>HHHHASILIDTSAWVEYFRATGSIAAVEVRRLLSEEAARIAMCEPIAMEILSGALDDNTHTTLERLVNGLPS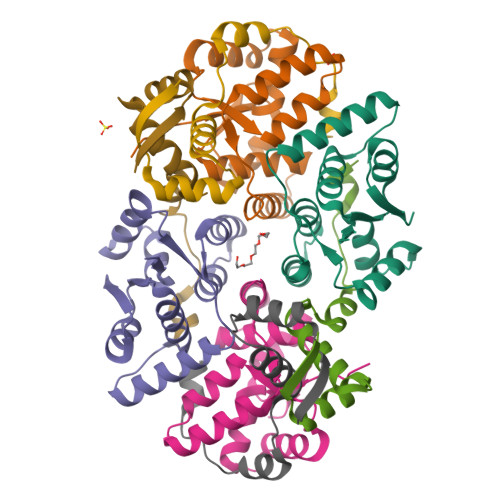LNVDDAIDFRAAAGIYRAARRAGETVRSINDCLIAALAIRHGARIVHRDADFDVIARITNLQAASFR[4x];>SRTNIDIDDELAAEVMRRFGLTTKRAAVDLALRRLVGSPLSREFLLGLEGVGWEGDLDDLRS[4x]> GAMVQISEVRGNTRDHRTAAHTHIKGLGLNSSGIAEKQAAGFVGQCAAREACGVVVDLIKAHKMAGRGVLLAGGPGTGKTALALAISQELGTKIPFCPITGSEIYSTEVKKTEVLMENFRRAIGLRVRETKDVYEGEVTEMTPEEAENPLGGYGKTISTLLIGLKSARGQKKLRLDPSIYEAIQKERVQVGDVIYIETNTGACKRVGRSDAYATEFDLEAEEYVPIPKGEVHKKKEIVQDVTLHDLDVANARPQGGQDIISMMGQLMKPKMTEITDKLRMEINKVVQKYINQGVAELIPGVLFIDEAHMLDIECFTYLNKALESPIAPIVVLASNRGIATIRGADDLKAAHGIPPDFLQRLLIIPTHPYEPDEIRRIVRIRAQTEGVQLTDAAVDRVAEHGVRISLRYCLQLLAPASILARVNGRTQVDVQDIAEAEELFLDARRSANILTSTGESGGLHGFIS;> GAMAAPLVTSVTETKELRGLNLIAAHSHIRGLGVDADTLEPRPSSQGLVGQEKARKAAAVVLEMIKQGKIAGRAVLIAGPPSTGKTAIAMGMAQSLGQDVPFTTLAASEIFSLEMSKTEALTQAFRKSIGVRIKEESEIMEGEVVEIQIDRSVTGGAKQGKLTIKTTDMEAIYDMGSKMIDAMTKERVMAGDIISIDKSSGKITKLGRSYARSRDYDAMGVDTKFLQCPEGELQKRKEVVHTVSLHEIDVINSRTQGFLALFSGDTGEIRSEIRDQINTKVAEWKEEGKAEIVPGVLFIDEVHMLDIECFSYINRALESDLAPIVIMASNRGVSRIRGTDYKSPHGLPLDFLDRVVIINTHPYTPDELRQILSIRAQEEEVDLTPDALALLTKIGQEAGLRYASNLITTSQLIAAKRRAKQVGVEDVQRSFKLFYDPARSVRFVQESEKRLIGNDGVVDFSYQGAAEAAAPTLPAAAPVDPVGGEKMDMS

Rvb1 and Rvb2 are highly conserved eukaryotic proteins, very similar to each other, that belong to the large AAA+ (ATPases associated with diverse cellular activities) superfamily of ATPases. Rvb1 and Rvb2 (also known as RuvBL1/RuvBL2, Pontin/Reptin, TIP49a/TIP49b) are necessary for cell viability and play essential roles in various complexes involved in fundamental processes such as transcription regulation, DNA damage response and apoptosis (via the chromatin remodelling complexes SWR1, INO80 and TIP60), maturation of small nuclear ribonucleoproteins, cellular development, cancer metastasis and regulation of mitosis. Domain II (DII) corresponds to an insertion of 160–170 amino acids in domain DI between the Walker A and B motifs that is unique to Rvb1 and Rvb2 in comparison with other AAA+ family members. Here, we report the crystal structure of the dodecameric Rvb1/Rvb2 complex from Chaetomium thermophilum (Ct) at 2.9 and 3 Å resolution in two nucleotide binding states (ADP/ADP and ADP/PP) together with two cryo-EM reconstructions of the same complex in the stretched and compact conformation at 21 and 12 Å resolution.

Therefore, the complex structure was solved using selenomethionine (SeMet) substituted proteins in a single anomalous dispersion (SAD) experiment and subsequently refined to Rwork/Rfree values of 23.0/25.6%. The Rvb1/Rvb2 complex crystallized in space group H32 with one Rvb1/Rvb2 heterodimer in the asymmetric unit. The SeMet crystals revealed density in Rvb1 that could be identified as ADP, whereas Rvb2 clearly shows two density peaks at the same position most likely corresponding to sulphates present in the crystallization solution and known to mimic phosphates. We will therefore refer to this state as ADP/PP. There are no obvious differences when comparing the Rvb1 nucleotide binding pocket in the ADP/ADP (native) dimer and in the ADP/PP (SeMet) dimer. In contrast, we observe subtle changes in the case of Rvb2. First, Arg399 in sensor II is interacting with the adenine in the ADP form and bends towards one of the sulphates in the PP state. Second, Asp298 in the Walker B motif flips towards the sulphate in the PP state. Finally, the “trans-arginine finger” Arg358 of Rvb1 that protrudes into the Rvb2 nucleotide binding pocket stabilizes both the ADP and the PP state. Despite some missing residues in the sulphate-bound Rvb2, this tail has a similar position as in the ADP-bound Rvb1.> AEIYNKDGNKLDVYGKVKAMHYMSDNASKDGDQSYIRFGFKGETQINDQLTGYGRWEAEFAGNKAESDTAQQKTRLAFAGLKYKDLGSFDYGRNLGALYDVEAWTDMFPEFGGDSSAQTDNFMTKRASGLATYRNTDFFGVIDGLNLTLQYQGKNENRDVKKQNGDGFGTSLTYDFGGSDFAISGAYTNSDRTNEQNLQSRGTGKRAEAWATGLKYDANNIYLATFYSETRKMTPITGGFANKTQNFEAVAQYQFDFGLRPSLGYVLSKGKDIEGIGDEDL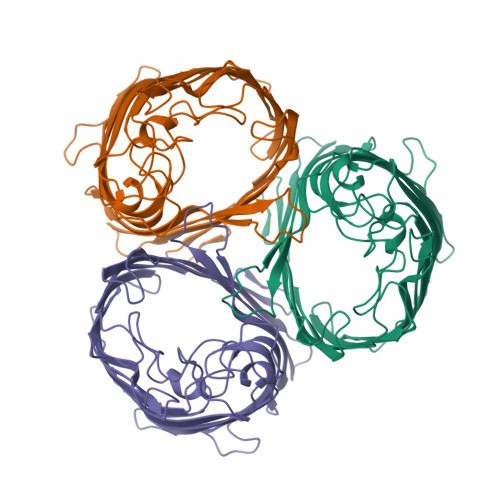VNYIDVGATYYFNKNMSAFVDYKINQLDSDNKLNINNDDIVAVGMTYQF> XSLSDKDKAAVRALWSKIGKSADAIGNDALSRMIVVYPQTKTYFSHWPDVTPGSPHIKAHGKKVMGGIALAVSKIDDLKTGLMELSEQHAYKLRVDPANFKILNHCILVVISTMFP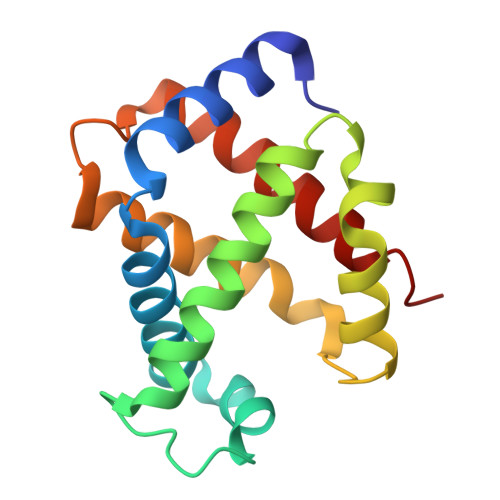KEFTPEAHVSLDKFLSGVALALAERYR>GHVAGPIAVGCYPALGPTILPSMLYAFTAEYPRASVEFREDTQNRLRTQLEGGELDVAIVYDLDLSPEWQTVPL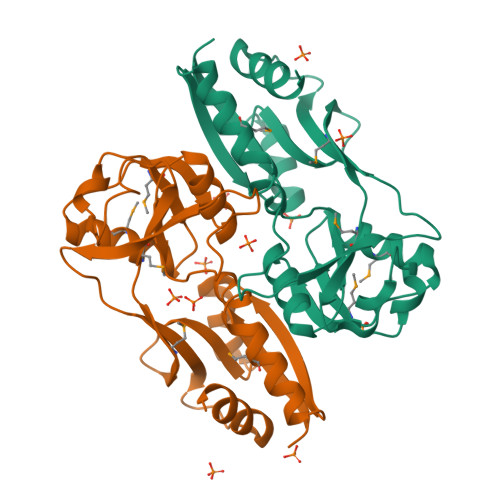MTREPMVVLGAEHPLAGVDGPVRLADLAEHPMVLLDAPPSTNHAMDVCREAGFAPRVAYRTANFETARAFVGRGLGWTLLLQRPRVDVTYEGLPVVVKPIAEPKPASVAVVVAWHQEATLSRVARAFIRFVTAGS[12x]> GPLPKPTLWAEPGSVITQGSPVTLRCQGSLETQEYHLYREKKTALWITRIPQ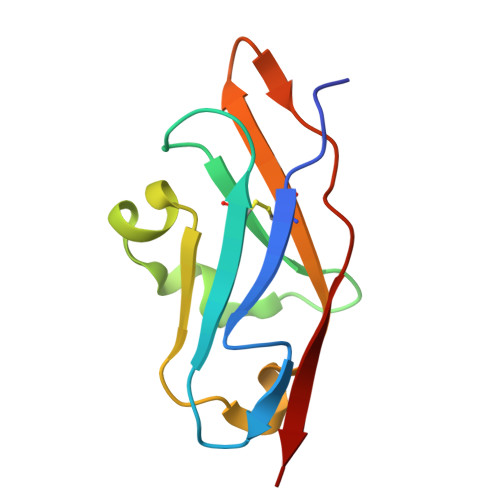ELVKKGQFPILSITWEHAGRYCCIYGSHTVGLSESSDPLELVVTG>HHHHHHIEGRMKPSPEILALRWKDTCAHYSPHEWVAARNVVTANKAALADYFYECMLADPNAAFFLSDQLVKTKLHASMQDWLESVYAAAPTEEYERTVAFQRKVGEVHAR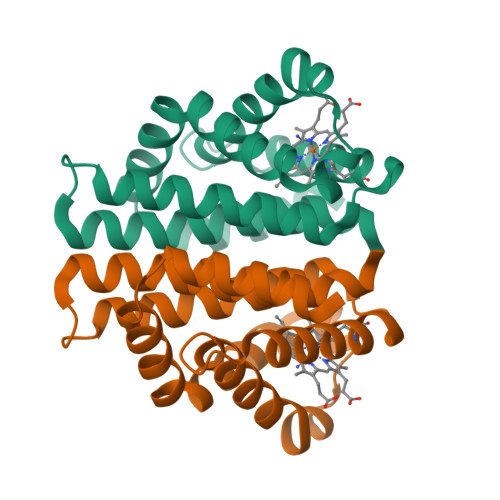IDIPVHLVTRGACALIRRICELLDRDASLSAAQAAATCRYVADVTMTAVEMMCHAYSVS[3x]3-({[(4-nitrophenyl)carbamoyl]amino}methyl)-1-(5-O-phosphono-beta-D-ribofuranosyl)pyridin-1-ium | C18 H22 N4 O10 P | 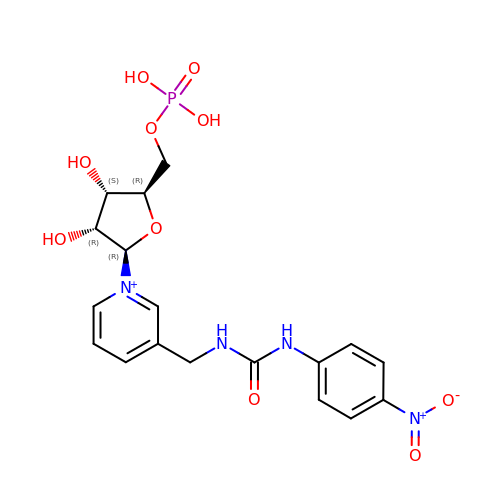OCUAXUHZRNUDEK-QBPKDAKJSA-O> GSVADIQQLEEKV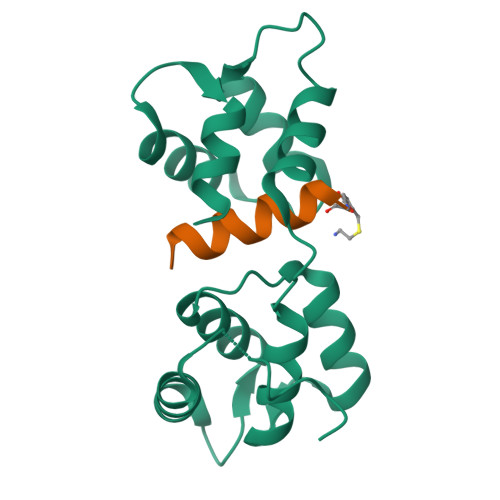DESDVRIYFNEKSSGGKISIDNASYNARKLGLAPSSIDEKKIKELYGDNLTYEQYLEYLSICVHDKDNVEELIKMFAHFDNNCTGYLTKSQMKNILTTWGDALTDQEAIDALNAFSSEDNIDYKLFCEDILQ;> GSLLRVQAHIRKKMV>[4x]EFYQQWQLKYPKLILREASSVSEELHKEVQEAFLTLHKHGCLFRDLVRIKGKDLLTP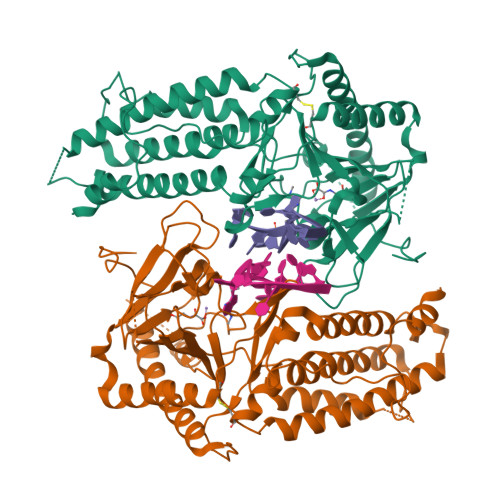VSRILIGNPGCTYKYLNTRLFTVPWPVKGSNIKHTEAEIAAACETFLKLNDYLQIETIQALEELAAKEKANEDAVPLCMSADFPRVGMGSSYNGQDEVDIKSRAAYNVTLLNFMDPQKMPYLKEEPYFGMGKMAVSWHHDENLVDRSAVAVYSYSCEGPEEESEDDSHLEGRDPDIWHVGFKISWDIETPGLAIPLHQGDCYFMLDDLNATHKHCVLAGSQPRFSSTHRVAECSTGTLDYILQRCQLALQNVCDDVDNDDVSLKSFEPAVLKQGEEIHNEVEFEWLRQFWFQGNRYRKCTDWWCQPMAQLEALWKKMEGVTNAVLHEVKREGLPVEQRNEILTAILASLTARQNLRREWHARCQSRIARTLPADQKPECRPYWEKDDASMPLPFDLTDIVSELRGQ>MSFPYFISPEQAMRERSELARKGIARAKSVVALAYAGGVLFVAENPSRSLQKISELYDRVGFAAAGKFNEFDNLRRGGIQFADTRGYAYDRRDVTGRQLANVYAQTLGTIFTEQAKPYEVELCVAEVAHYGETKRPELYRITYDGSIADEPHFVVMGGTTEPIANALKESYAENASLTDALRIAVAALRAGSADTSGGDQPTLGVASLEVAVLDANRPRRAFRRITGSALQALLVDQESPQSDGESSG[14x];>ATIVALKYPGGVVMAGDRRSTQGNMISGRDVRKVYITDDYTATGIAGTAAVAVEFARLYAVELEHYEKLEGVPLTFAGKINRLAIMVRGNLAAAMQGLLALPLLAGYDIHASDPQSAGRIVSFDAAGGWNIEEEGYQAVGSGSLFAKSSMKKLYSQVTDGDSGLRVAVEALYDAADDDSATGGPDLVRGIFPTAVIIDADGAVDVPESRIAELARAIIESRSGADTFGSDGGEK[14x]

The Mycobacterium tuberculosis (Mtb) proteasome system selectively degrades damaged or misfolded proteins and is crucial for the pathogen’s survival within the host. Mtb 20S core particle features homoheptameric rings in a conserved α7-β7-β7-α7 configuration. These rings assemble to form three interconnected compartments: two antechambers formed by α7-β7 and a central degradation chamber. Stacked β-rings enclose the degradation chamber where active sites containing the catalytic triad of βT1, βD17, and βK33 proteolyze substrates.

Notably, 20SβT1A has a slightly higher RMSD value of 0.63 Å compared to the 20SOG variant (RMSD 0.22 Å) and the ixazomib-bound 20SWT variant (RMSD 0.35 Å), highlighting subtle structural differences between them. A comparison of Cα RMSD values calculated separately for the α- and β-subunits showed that conformational changes in the β-subunit primarily account for the observed RMSD deviation in the 20SβT1A variant. While the overall arrangement of the catalytic residues within the 20S CP is essentially unchanged, we noticed small but clear differences in the structure of the 20SβT1A variant. Notably, the longitudinal axis of the helix formed by residues βA49-E70, hereafter referred to as switch helix I, shifts by 4 degrees in 20SβT1A compared to all the other 20S variants. This results in the displacement of switch helix I by 4.7 Å, which in turn shifts an upstream β-strand and short loop containing residues βA46, βG47, βT48, and βA49, which form the back of the S1 pocket. The altered position of switch helix I is stabilized through the formation of a new hydrogen bond between the backbone carbonyl of βG47 and Nε of βK33. The helix formed by residues βF76-Q96, hereafter referred to as switch helix II, is unchanged in this structure. Of note, switch helix I shifts by 4.7 Å in the refined atomic model of the 20SβT1A variant, while switch helix II undergoes no structural changes in the consensus map as this represents the average state of the particles in the dataset. In contrast to the βT1A variant structure reported by Li et al., which was crystallized with the β-propeptide present and adopts the canonical state of the 20S, our cryo-EM structure of the 20ST1A variant lacks the β-propeptide, potentially accounting for the observed conformational differences.DSR2, a Sir2 domain-containing protein, protects bacteria from phage infection by hydrolyzing NAD+. The enzymatic activity of DSR2 is triggered by the SPR phage tail tube protein (TTP), while suppressed by the SPbeta phage-encoded DSAD1 protein, enabling phages to evade the host defense. The protomer structure of DSR2 revealed an architecture that consists of an N-terminal Sir2 domain (residues 1–298) and a long C-terminal helical region (residues 299–1005). The Sir2 domains of two side-by-side DSR2 dimers contact each other to assemble into a head-to-head rod-shaped homo-tetramer of DSR2.

In comparison with that of DSR2 alone, the map of the DSR2-DSAD1 complex displays an extra density on the C-terminal cavity of DSR2, which corresponds to DSAD1. However, the resolution of DSAD1 and its binding region in DSR2 is relatively low, posing challenges for model building. By employing local refinement focused solely on the DSR2-DSAD1 interaction region, the resolution for this specific area was improved to 3.2 Å. The sidechains of the majority of DSAD1 residues were distinctly visible, enabling successful de novo construction of the atomic model for DSAD1 and the entire DSR2-DSAD1 complex. The DSAD1 structure comprises one α-helix and eight β-strands, forming three intertwined β sheets, which deviates significantly from the initially predicted AlphaFold2 model. In the interface 1, a long flexible loop between β5 and β6 of DSAD1 is embedded into the cavity of DSR2, while in the interface 2, the body of DSAD1 locates on the top of the cavity. The aromatic sidechain of F59 from DSAD1 inserts into a hydrophobic pocket constituted by the sidechains of I918, W919, L922 and L966 from DSR2. The side chain of N21 from the DSAD1 establishes two hydrogen bonds with the nearby sidechains of S957 and K960 from DSR2. The first helix of the HEAT repeat domain and the following repeat R1 directly contact DSAD1. This region contributes a β strand that is disordered in apo structure to form a three stranded β sheet with β1 and β2 of DSAD1, rendering the partially opened cavity closed.

>MVKVDLESKRYGEKLKEVFLMLDNNVVECIKEITESSRNGKLVFFVGAGVSTLSDYPQWWRLVDKYHEELYGSPKKGNYSSDEYLRIPQIFYNVKGEMAFDGILKDFFQVDKPTNPIHDKILAMNPAHVITTNYDNLIDTACWKRGKYFSVISAEEDVANATSSRYLLKVHGDFRKGFKGENVVLKEDDYLNYDQNYPLISNLMKTIIATHTIVFIGYGLGDYNINMLLNWVRKLQKDSFHKPFFIRTDPSPIENETLIYYENKGLRIIDAASLIDSNEYDYLERYSAVMDLLIESQENKFITKDDEVIDYIYGKISPLFALQYIRKIDLKHVFEYDYHFEVNGTVVRHKNKGFGYMERFFELKESCDERSKLSKKQYERFNALFNFFEKNGVICMAKDAGTLNTSIEINSLAYHGKYDVMKKFIEEQSVSIEDDYKKAFFLACLGRWEESYDLYSNIILNSIDESNGCVYYLSQINRYRIYQSITQAVTQFNGLGLLTFGRHYKPFTDEFLARIEREMTNFNIDDLFNGMPFEFQKKYKILEFLSDNQFLYDDTVKLFELTNKVRSEMSEGSYSFGMSSDIVVLLRLYDNLRFLYENCLWSVSFHEFHQYIRNSMSLLIEKAEYERTRDIDELGFSFFGKKSGFFMEYYDFVNISRHFKIDDIKNLERSCSIDKIRFGEQEKIEEYLVGIAEEITKQFSANGMNVVFYTQFISEAKAALYFAKYVKLSEEGLGKIVKALLFYFPERDLDIGKRYVWLERLTKCNELPKSIISIIDDFLVLQAEKHIDQNYSEVSSNGLYSRDYGALIKHFEKNFISKRLSEITLCLTQDKQKQIDFLFKLLPLLSTNAKSHLLSFKSVENINDLMNGIRIGLIDEFTPEHEELIIEYLETRKVNYIVEKEKGIQTFSSNDYMSTFGIWYFLEEINNSKMEEFIGMDDQYDFFVDPENFDYKKFIPSWLKNYNDKLLGKIAGNKHMKHHVIEVLKERVKNSNDKRYLEILMNYFI[2x];> MIEIFKDTGATHDLVYHSKINTFVWDVEFDIVLSDSKELNKCYFVKCFNPYRINGKCDFAVSSIDIFSEGKRLLIENEFNFKITKAVHVATSKDVTEIVLHLSERISSPFPIVKEVVYLD8-hydroxy-2-methylquinoline-6-carboxamide | C11 H10 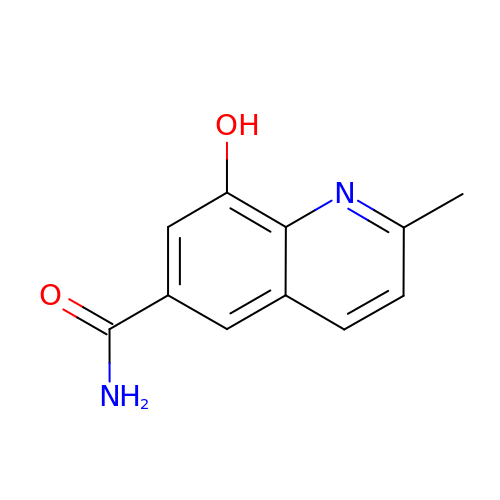N2 O2 | CTRBRVRHXAPYCD-UHFFFAOYSA-N2-amino-4,5-dimethoxybenzoic acid | C9 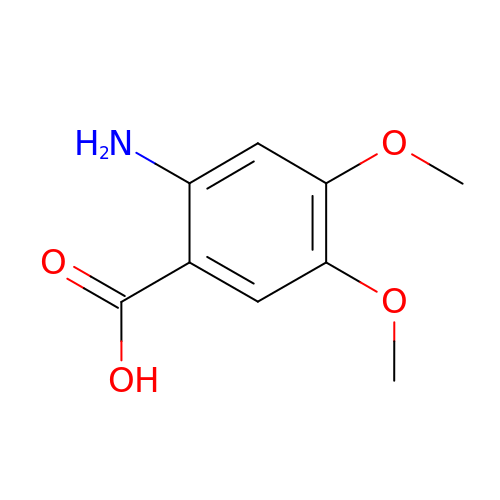H11 N O4 | HJVAVGOPTDJYOJ-UHFFFAOYSA-N> SMHDPIPTIAFPDGRKVPALGQGTWRMGENRAKTADEVRSLQTGLDLGMTLIDTAEMYGDGAAERIVGEAIKGRRDEAFVVSKVLPSNASRAGTVAACERSLRNLGIDCVDLYLLHWRGGYPLAETVAAFEELKKAGKIRAWGVSNFDVDDMEELSAVPDGGNVAANQVLYNLARR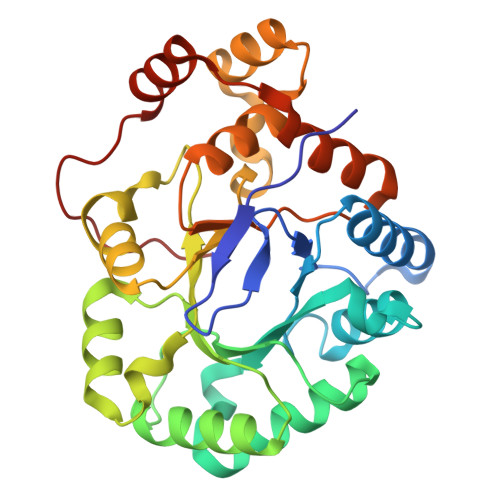GIEFDLLPRCRAQGVPVMAYSPLDEGRLLHDADLIHIAKAHQATPAQVALAFLKTCSGVISIPKTGSPERARENRDAMDIHLTTENLAELDRHFPPPRRKTRLEVI BIS(5-AMIDINO-2-BENZIMIDAZOLYL)METHANE KETONE | C17 H16 N8 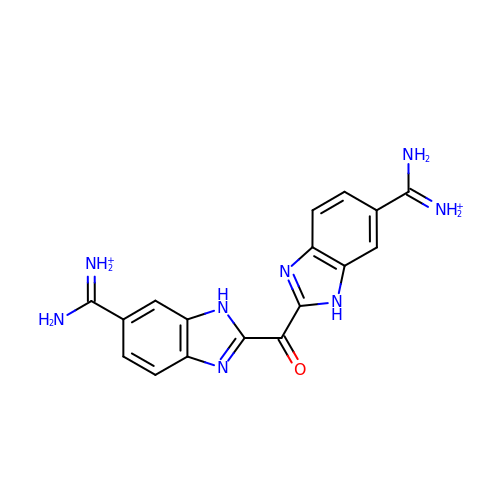O | VVVXDHROXQUONB-UHFFFAOYSA-P>[8x]MTLVHNWHLGRRMEYPYFESRPKHQFAAVFNINRCIACQTCTMACKSTWTFNKGQEFMWWNNVETKPYGGFPQSWDVKTLKLIDSPDNIWYTDDKDKETSQYGTGAPYGTYEGDTIFEVAKKKNINQWAVGYIPEDKEWRSPNFGEDTAKSSNQPGEYSTLPEHSRWFFYLQ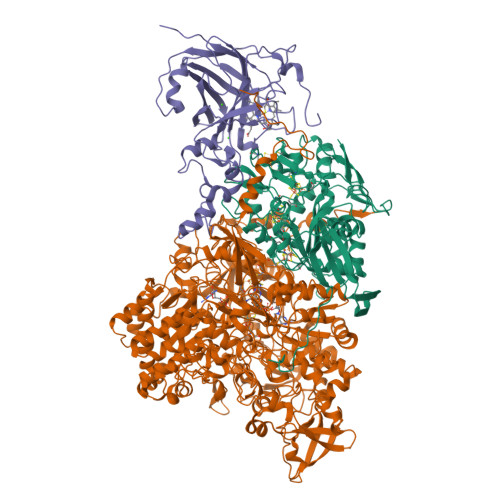RICNHCTYPGCLAACPRKAIYKRKEDGIVLIDQKRCRGYRKCVEQCPYKKPMYRGLTRVSEKCIACYPRIEGRDSLTDGRPMETRCMSACVGQIRLQGFLDDNPKNPITWLIRHQKIALPLYPQFGTEPNIYYIPPRWAPRAYLRQMFGPGVDEAIEKFMVPSRELLAVMSLFRMTQTIVYEYKIEEGPKVFETEIHGKKFTMYNDTVIGFGEDGKEVVRTTVEEPIHIRPDKHYNSI;>[8x]MKLTRRAFLQVAGATGATLTLAKNAMAFRLLKPAVVVDNPLDTYPDRRWESVYRDQYQYDRTFTYCCSPNDTHACRIRAFVRNNVMMRVEQNYDHQNYSDLYGNKATRNWNPRMCLKGYTFHRRVYGPYRLRYPLIRKGWKRWADDGFPELTPENKTKYMFDNRGNDELLRASWDEAFTYASKGIIHITKKYSGPEGAQKLIDQGYPKEMVDRMQGAGTRTFKGRGGMGLLGVIGKYGMYRFNNCLAIVDAHNRGVGPDQALGGRNWSNYTWHGDQAPGHPFSHGLQTSDVDMNDVRFSKLLIQTGKNLIENKMPEAHWVTEVMERGGKIVVITPEYSPSAQKADYWIPIRNNTDTALFLGITKILIDNKWYDADYVKKFTDFPLLIRTDTLKRVSPKDIIPNYKLQDISDGPSYHIQGLKDEQREIIGDFVVWDAKSKGPKAITRDDVGETLVKKGIDPVLEGSFKLKTIDGKEIEVMTLLEMYKIHLRDYDIDSVVSMTNSPKDLIERLAKDIATIKPVAIHYGEGVNHYFHATLMNRSYYLPVMLTGNVGYFGSGSHTWAGNYKAGNFQASKWSGPGFYGWVAEDVFKPNLDPYASAKDLNIKGRALDEEVAYWNHSERPLIVNTPKYGRKVFTGKTHMPSPTKVLWFTNVNLINNAKHVYQMLKNVNPNIEQIMSTDIEITGSIEYADFAFPANSWVEFQEFEITNSCSNPFIQIWGKTGITPVYESKDDVKILAGMASKLGELLRDKRFEDNWKFAIEGRASVYINRLLDGSTTMKGYTCEDILNGKYGEPGVAMLLFRTYPRHPFWEQVHESLPFYTPTGRLQAYNDEPEIIEYGENFIVHREGPEATPYLPNAIVSTNPYIRPDDYGIPENAEYWEDRTVRNIKKSWEETKKTKNFLWEKGYHFYCVTPKSRHTVHSQWAVTDWNFIWNNNFGDPYRMDKRMPGVGEHQIHIHPQAARDLGIEDGDYVYVDANPADRPYEGWKPNDSFYKVSRLMLRAKYNPAYPYNCTMMKHSAWISSDKTVQAHETRPDGRALSPSGYQSSFRYGSQQSITRDWSMPMHQLDSLFHKAKIGMKFIFGFEADNHCINTVPKETLVKITKAENGGMGGKGVWDPVKTGYTAGNENDFMKKFLNGELIKVDA;>[8x]MKKFYRLLGSSSVALLGCLFLSVALCIAEEAEGVKGVAEEELTPAKEVLNVKYMQIDVPAHITVGALEGAFKNAEGVQVKLQKQDKAFPNGGGSVNSAEIKAIHDGITIYFQVIWDDATDNKQAIATQEFRDGAALMFPLGKITISPEEPFSPRMGDRQKPVNLWHWKADWEADLLATGGIEECPARYPNMHDDFSTNPHSVNYHKGVIQSAAELSGGYAAHNLLSLPRGRAVEDLNAEGFGTLTSQDHQDVDGCSKFENKKWTVVFCRSLNTGDPLDVQFVPGESTYFNMAVWNGDREDRNGQKNISIQWHPLSLERIAWQ> MMEQVCDVFDIYAICACCKVESKNEGKKNEVFNNYTFRGLGNKGVLPWKCISLDMKYFRAVTTYVNESKYEKLKYKRCKYLNKETVDNVNDMPNSKKLQNVVVMGRTNWESIPKKFKPLSNRINVILSRTLKKEDFDEDVYIINKVEDLIVLLGKLNYYKCFILGGSVVYQEFLEKKLIKKIYFTRINSTYECDVFFPEINENEYQIISVSDVYTSNNTTLDFIIYKKTNNKMLNEQNCIKGEEKNNDMPLKNDDKD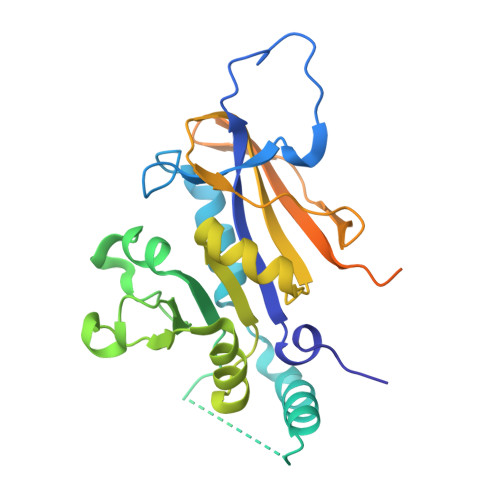TCHMKKLTEFYKNVDKYKINYEN> DTSTWFI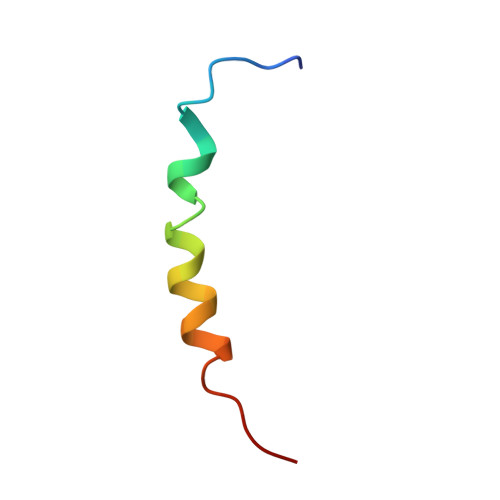TITSMIMTLFILFQLKISNYSYP>[2x]MKEITLTIDGKVCKGVQGDTILDVANKNDVYIPTLCYQKGLTPIGACRMCVVQLEGNPKMLPSCTTPAQDGMVVVTKNEKLKDYRRQILELLFAGRNHFCMYCSQSGDCELQRLAIEHEMDSVRFPYLYEDFEVDATDPNLMMDHNRCVLCQRCIRTCSEIVGAHTLDLERRGWQAKVIADLGKRLRESDTCVNCGACAQSCPTGTITIREFAYRGRRSECDAVVESVCPLCAVGCKIKTYVRTGSIVRVEGTGVEEPDGGQLCHMGRWWLPESTERERVTVPLIREGASYREATWEEALALASAEFKKAYDQEKAGAILSSLCTDEELTLFSALFRNALKMKHIDTFDGDIIRGFFKGFMPFREQGVRPFTAAHHILDSDLIITMFADPQKEAPVVASYIRVACLHRNAKLMNLSYGPSPFPGLVDLDIRLPEGQAVPKALSNLAEIIGKISLGPSDMASFGEFEAGAGKALSSYRESIEESARAMGLDPKIAEEVALMLISARRPIFIIGGRATKSHELVTAACNLAVASKAFFEDGLGVVPLLVSANSLGARNTVVSENPWLGRERRDFLYVFSTAMVPEEEEILAAISATRFVVVQTPFKVRPLVNLADILLPAPAWYERSGHFCTIEGERRKLNTIVPPKGEIKSLHYVMDEFAKKLGVKLERPEVSPCEEIFKSQLRASEARIVTL;>[2x]MAIYRAHVLVCRGTGCTASGAPGVMKAFKEELAKKGLDREVMLVETGCHGMCEMGPVVVVYPEGAFYCRVTPEDVPEIVEEHLYKGRIVQRLLYTVPEDMEKVPYYKDIPFYSKQHRIVLSNCGYIDPEKIEEYIARDGYMALGKALLEMTPEEVLEEVKKSGLRGRGGAGFPTGLKWEFAKKASGDKKYVICNADEGDPGAFMDRSTLEGDPHSVIEGMTIGAYVIGADEGYIYCRAEYPLAIKRLKIAIAQAEEMGLLGDHIMGTNFSFHLHLKEGAGAFVCGEETALMASIEGRRGMPRPRPPFPAQHGLWGKPTNINNVETWANVPRIILNGADWFASMGTEKSKGTKIFALTGKITNTGLIEVPMGITIREIIYELGGGILNGKEFKAVQIGGPSGGCLTKEHLDLPIDYESLTAAGAIMGSGGLVVMDEDTCMVDVAKFFLEFTQRESCGKCVPCREGTKQMLLMLQKICNGEGTMDDLSKLEELAHMVKETSLCGLGQTAPNPVITTIRYFRDEYVAHIKDKRCPAKICPALIKYVVDPEKCRKCGLCARNCPVKCISGDRQTPYLINQEKCIKCGTCMQVCPFGAIGKV;>MALSTVDVVEKVKEIVAPWKGKQGGLIPILQEVQRELGYLPEEALLTISRELKMPKAEVYGVATFYAQFHLKPRGRHVIRVCRGTACHVRGSLQILEKVKQMLGIEENETTDDLRFTLEPVACLGACGLAPVMMVDEDTHGRMTPDKIQAILDKYQ[2x];>MTEVFKLEINPVTRIEGHGKITVMLDESGHVRETRFHVTQYRGFEVFTHGRDFREMPVITPRICGI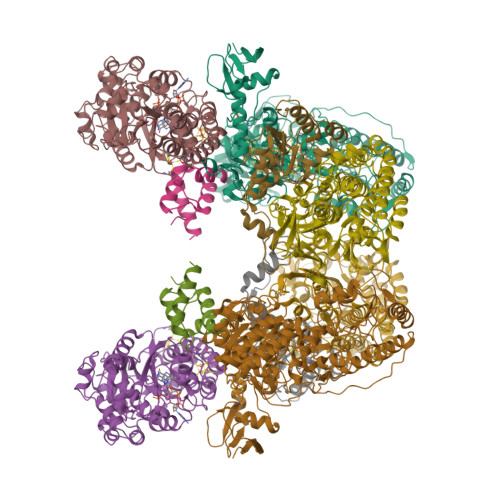CPVSHHLASAKACDEILGVTITPAAHKLRELMHMGQIVQSHALSFFHLSSPDILWGFDAPVKIRNVAGLVDRYPELAKKGIMLRKFGQEIIKTLGGKKIHPWHSIPGGVNRSLTPQERDAIAAQLPEMKSIAMEAIKLIKDYLQEGGEELKEFATLDTAYMGLVRDGYLELYDGEVRIKAPRGRILDQFDPKDYLDHIGEHVEPWSYLKFPFYKALGFPHGSYRVGPLARLNAADAVSTPEASKEFALYKEMGEDGIVPYTLYYHYARLIEALYGLERIEQLLADPDITSSDLRVTSKEINPEGIGVIEAPRGTLIHHYQVNESGVITKVNLIVATGHNNFAMNKGVEMVAKKYITGTNVPEGVFNRLEHVIRAYDPCLSCSTHAVGKMPLKLELVGPTGEILKEVTRD[2x];>MAKAKVATFWLEACAGCHMSFLDLDERLIDLFQNVEILFSPIVDAKDIPNIDVGVLSGGLGNVEEVELAKKMRERCKYLVAWGDCAVFGGINCMRNFIPKDVVLREGYIETASTVNPQGIVPSEDIPELLPRALPIDYEVKVDVYVPGCPPDADTIYYVFKELLAGRVPKVPSEMMRYD[2x]>[6x]MSDQPIIRRRQVKTGISDARANNAKTQSQYQPYKDA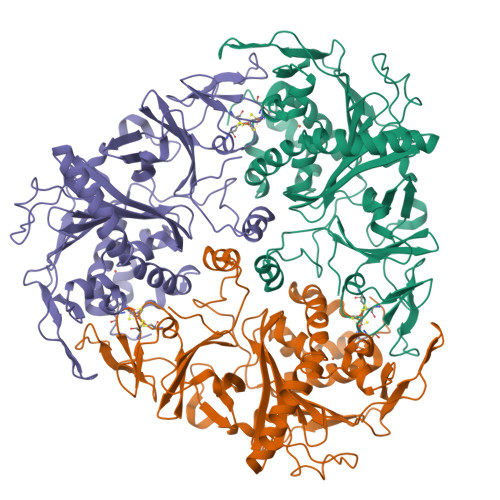AWGFINHWYPALFTHELEEDQVQGIQICGVPIVLRRVNGKVFALKDQCLHRGVRLSEKPTCFTKSTISCWYHGFTFDLETGKLVTIVANPEDKLIGTTGVTTYPVHEVNGMIFVFVREDDFPDEDVPPLAHDLPFRFPERSEQFPHPLWPSSPSVLDDNAVVHGMHRTGFGNWRIACENGFDNAHILVHKDNTIVHAMDWVLPLGLLPTSDDCIAVVEDDDGPKGMMQWLFTDKWAPVLENQELGLKVEGLKGRHYRTSVVLPGVLMVENWPEEHVVQYEWYVPITDDTHEYWEILVRVCPTDEDRKKFQYRYDHMYKPLCLHGFNDSDLYAREAMQNFYYDGTGWDDEQLVATDISPITWRKLASRWNRGIAKPGRGVAGAVKDTSLIFKQTADGKRPGYKVEQIKEDH> MATAQSNSPRVFCIGTADTKFDELRFLSEHVRSSLNSFSNKSSFKVGVTVVDVSTSWKETNSCADFDFVPSKDVLSCHTLGEETMGTFADIRGLAIAIMSKALETFLSIANDEQNLAGVIGLGGSGGTSLLSSAFRSLPIGIPKVIISTVASGQTESYIGTSDLVLFPSVVDICGINNVSKVVLSNAGAAFAGMVIGRLESSKEHSITNGKFTVGVTMFGVTTPCVNAVKERLVKEGYETLVFHATG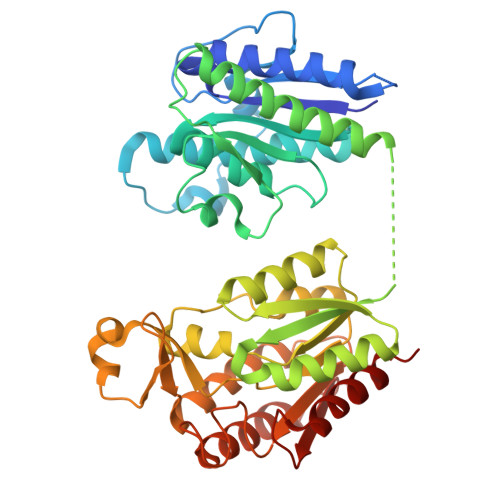VGGRAMEDLVRGGFIQGVLDITTTEVADYVVGGVMACDSSRFDAILEKKIPLVLSVGALDMVNFGPKTTIPPEFQQRKIHEHNEQVSLMRTTVGENKKFAAFIAEKLNKASSSVCVCLPEKGVSALDAPGKDFYDPEATSCLTRELQMLLENNERCQVKVLPYHINDAEFANALVDSFLEISPK> ADRQQYLRQEVLRRAEATAASTSRSLALMYESEKVGVASSEELARQRGVLERTEKMVDKMDQ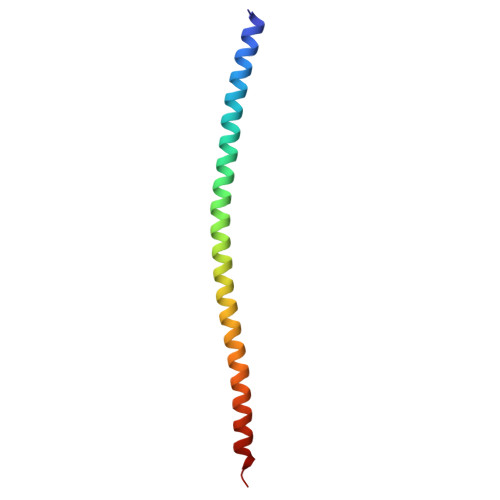DLKISQKHINSIKSVF> NIPFTDNLLFSGQVLYGDGRLTAKNHQLV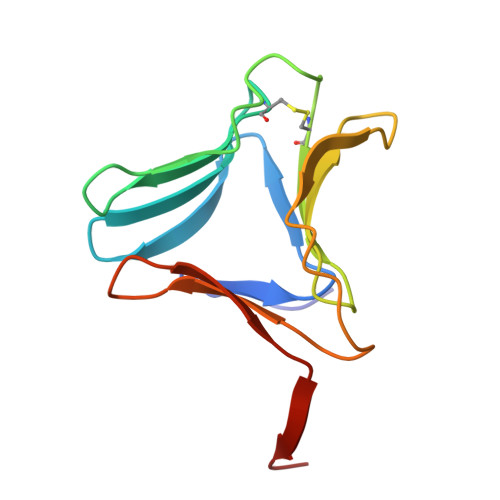MQGDCNLVLYGGKYGWQSNTHGNGEHCFLRLNHKGELIIKDDDFKTIWSSNSSSKQGDYVLILRDDGFAVIYGPAIWETSA>[2x]MRSHHHHHHGPGLVPRGSKTAAPVNALVSHLLVVEPEKLYAMPDPAGPDGHLPAVATLCDLFDREIVVTISWAKSIPGFSSLSLSDQMSVLQSVWMEVLVLGVAQRSLPLQDELAFAEDLVLDEEGARAAGLGELGAALLQLVRRLQALRLEREEYVLLKALALANSDSVHIEDAEAV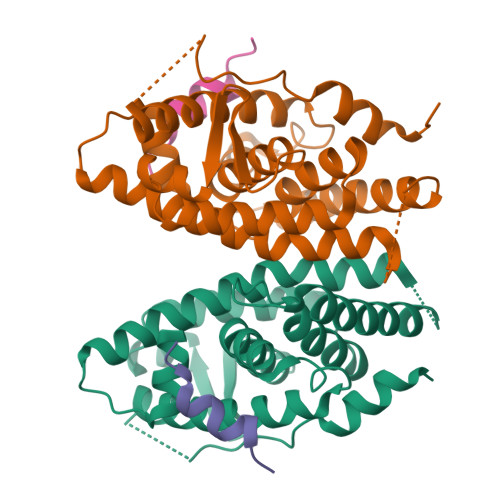EQLREALHEALLEYEAGRAGPGGGAERRRAGRLLLTLPLLRQTAGKVLAHFYGVKLEGKVPMHKLFLEMLEAMMD;>[2x]QQQKPQRRPCSELLKYLTTNDD> AELVRTDSPNFLCSVLPSHWRCNKTLPVAFKVVALGEVPDGTVVTVMAGNDENYSAELRNASAVMKNQVARFNDLRFVGRSGRGKSFTLTITVFTNPPQVATYHRAIKVTVDGPREPRRHRQKLDDSKPSLFSDRLSD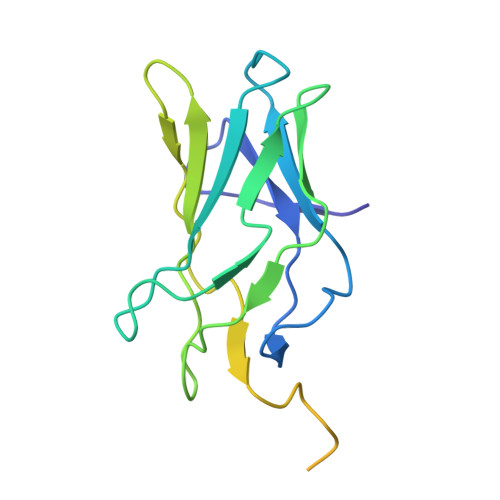LGRIPHPSMRVGVPPQNPRPSLNSAPSPFNPQGQSQITD> GTTPNSEGWHDGYYYSWWSDGGGDSTYTNNSGGTYEITWGNGGNLVG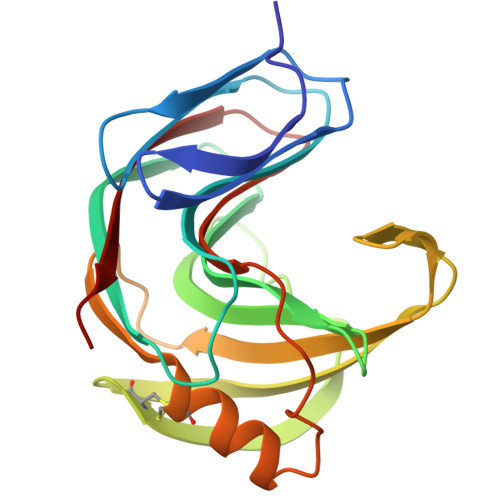GKGWNPGLNARAIHFTGVYQPNGTSYLSVYGWTRNPLVEYYIVENFGSSNPSSGSTDLGTVSCDGSTYTLGQSTRYNAPSIDGTQTFNQYWSVRQDKRSSGTVQTGCHFDAWASAGLNVTGDHYYQIVATEGYFSSGYARITVADVG>[3x]MVQTSFEHHHHHHSAGENLYFQGAQISMRLYSNRDRPNHLGPLALERLARVDDVVAQPARQPEDGFAASEDSLLGDVEEYARLFTRFLDGPVAPLGDAIPDDPARRAENLKASAYFLDASMVGICRLDPDDRAGDCDPSHTHALVFAVQFGREPEAGEAGAEWIRGTNAARTDMRCAEIAAILSGYVRWMGFPARGHFSGDAQVDLARLAVRAGLARVVDGVLVAPFLRRGFRLGVVTTGYALAADRPLAPEGDLGETAP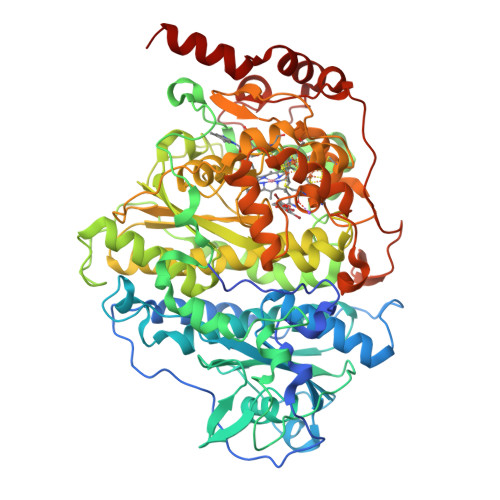EVMLGIDGTRPGWEDAEEEKRPLHMGRYPMETIRRVDEPTTLVVRQEIQRVAKRGDFFKRAEAGDLGEKAKQEKKRFPMKHPLALGMQPLIQNMVPLQGTREKLAPTGKGGDLSDPGRNAEAIKALGYYLGADFVGICRAEPWMYYASDEVEGKPIEAYHDYAVVMLIDQGYETMEGASGDDWISASQSMRAYMRGAEIAGVMAAHCRRMGYSARSHSNAHSEVIHNPAILMAGLGEVSRIGDTLLNPFIGPRSKSIVFTTDLPMSVDRPIDFGLQDFCNQCRKCARECPCNAISFGDKVMFNGYEIWKADVEKCTKYRVTQMKGSACGRCMKMCPWNREDTVEGRRLAELSIKVPEARAAIIAMDDALQNGKRNLIKRWWFDLEVIDGVAGAPRMGTNERDLSPDRGDKIGANQKLAMYPPRLQPPPGTTLDAVLPVDRSGGLAEYAAAETPAAARARLKSSAG>[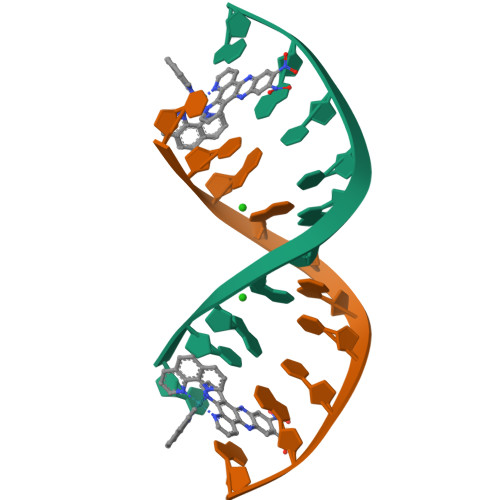2x]TCGGCGCCGA(3S,7R,11E)-7,14,16-trihydroxy-3-methyl-3,4,5,6,7,8,9,10-octahydro-1H-2-benzoxacyclotetradecin-1-one 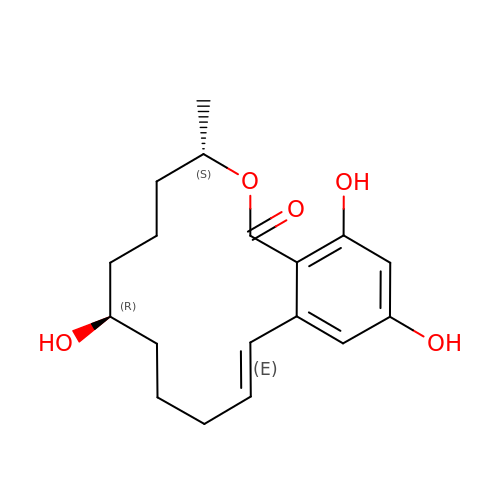| C18 H24 O5 | FPQFYIAXQDXNOR-QDKLYSGJSA-N>MANKDGPVCLQVKPC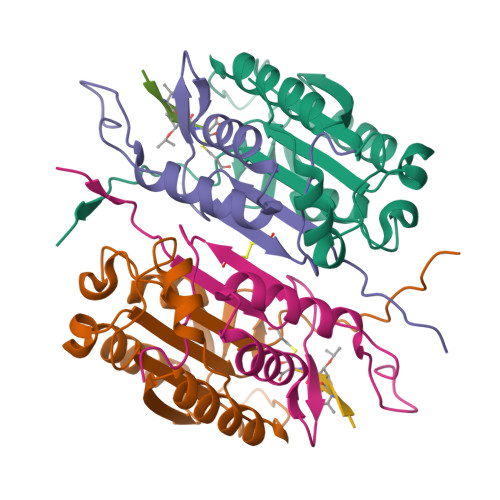TPEFYQTHFQLAYRLQSRPRGLALVLSNVHFTGEKELEFRSGGDVDHSTLVTLFKLLGYDVHVLCDQTAQEMQEKLQNFAQLPAHRVTDSCIVALLSHGVEGAIYGVDGKLLQLQEVFQLFDNANCPSLQNKPKMFFIQACRGDETDRGVDQQD[2x];>MAGKEKLPKMRLPTRSDMICGYACLKGTAAMRNTKRGSWYIEALAQVFSERACDMHVADMLVKVNALIKDREGYAPGTEFHRCKEMSEYCSTLCRHLYLFPGHPPTAAALEHHHHHH[2x]> SEGSTGTPRGSGSEDSFVKRARATEDFFVR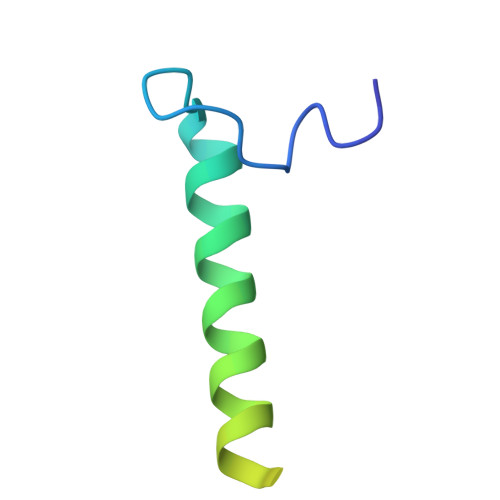QREKEQLRHLKEQLEKQRKKIDSLENKIDSMTK>[2x]MNKIFIYAG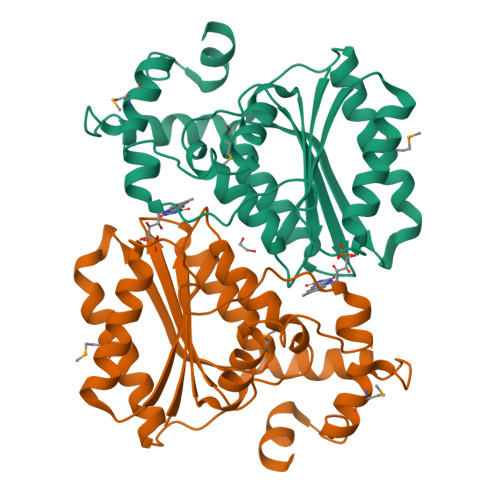VRNHNSKTLEYTKRLSSIISSRNNVDISFRTPFNSELEISNSDSEELFKKGIDRQSNADDGGVIKKELLESDIIIISSPVYLQNVSVDTKNFIERIGGWSHLFRLAGKFVVTLDVAESNGSDNVSEYLRDIFSYMGGQILHQVSITNSLKDIAEAQLMEATYKIEDVLEGKIKYKTTDYQERAYQTLKLILENYDSEHFEKMYWEKKRLFEANSLEEWYYVENIKLEHHHHHH>[8x]MVTSETV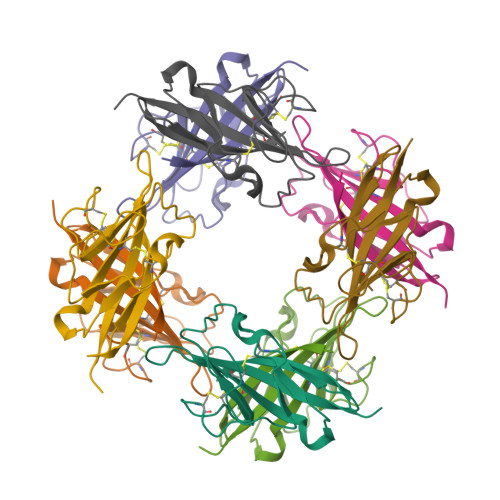VTEVLGHRVTLPCLYSSWSHNSNSMCWGKDQCPYSGCKEALIRTDGMRVTSRKSAKYRLQGTIPRGDVSLTILNPSESDSGVYCCRIEVPGWFNDVKINVRLNLQRA> KETAAA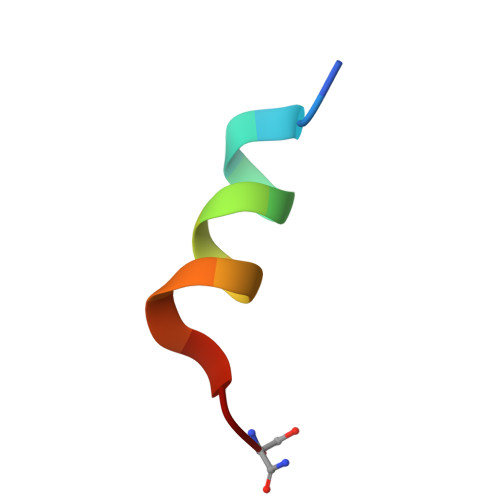KMERQHLDS>[3x]SMDPKYQRVELNDGHFMPVLGFGTYAPPEVPRNRAVEVTKLAIEAGFRHIDSAYLYNNEEQVGLAIRSKIADGSVKREDIFYTSKLWCTFFQPQMVQPALESSLKK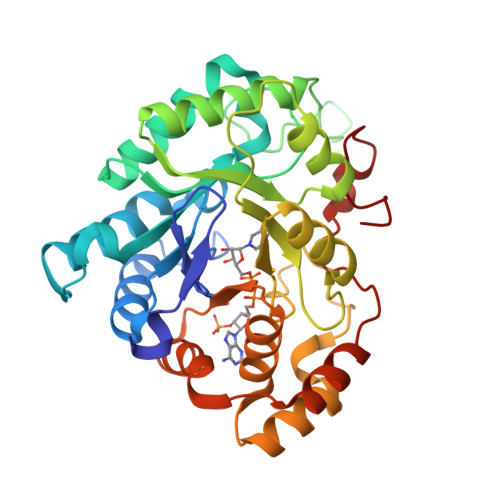LQLDYVDLYLLHFPMALKPGETPLPKDENGKVIFDTVDLSATWEVMEKCKDAGLAKSIGVSNFNYRQLEMILNKPGLKYKPVCNQVECHPYLNQSKLLDFCKSKDIVLVAHSALGTQRHKLWVDPNSPVLLEDPVLCALAKKHKRTPALIALRYQLQRGVVVLAKSYNEQRIRENIQVFEFQLTSEDMKVLDGLNRNYRYVVMDFLMDHPDYPFSDEY> MGTEFNGLFDEWAHTYDSFVQGEDIQYKEVFAHYEDILEDVVNKSFGNVLEFGVGTGNLTNKLLLAGRTVYGIEPSREMRMIAKEKLPKEFSITEGDFLSFEVPTSIDTIVSTYAFHHLTDDEKNVAIAKYSQLLNKGGKIVFADTIFADQDAYDKTVE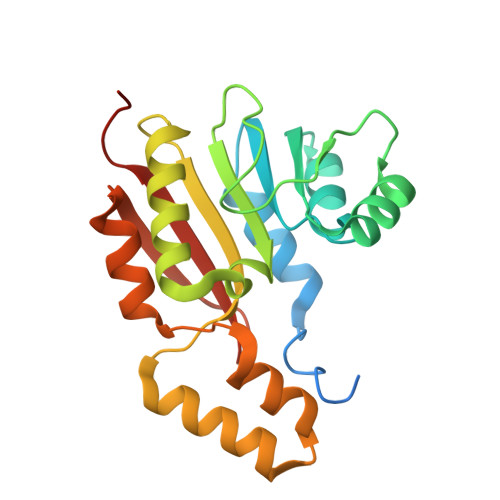AAKQRGFHQLANDLQTEYYTRIPVMQTIFENNGFHVTFTRLNHFVWVMEATKQLEHHHHHH> SQANLMRLKSDLFNRSPMYPGPTKDDPLTVTLGFTLQDIVKVDSSTNEVDLVYYEQQRWKLNSLMWDPNEYGNITDFRTSAADIWTPDITAYSSTRPVQVLSPQIAVVTHDGSVMFIPAQRLSFMCDPTGV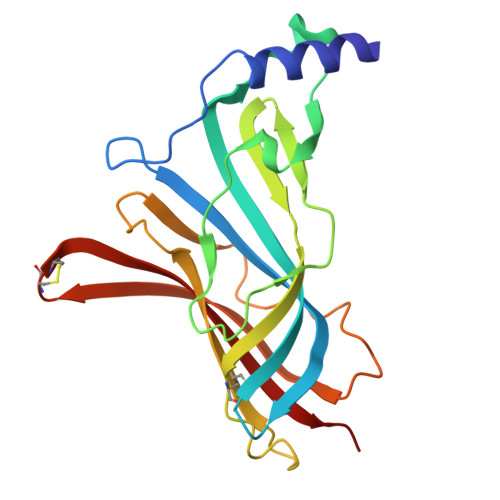DSEEGVTCAVKFGSWVYSGFEIDLKTDTDQVDLSSYYASSKYEILSATQTRQVQHYSCCPEPYIDVNLVVKFRERR The solute carrier 13 (SLC13) family comprises electrogenic sodium ion–coupled anion cotransporters, segregating into sodium ion–sulfate cotransporters (NaSs) and sodium ion–di- and–tricarboxylate cotransporters (NaDCs). NaS1 and NaDC1 regulate sulfate homeostasis and oxidative metabolism, respectively. From an overall view, both the NaDC1 and NaS1 form a homodimer, and each protomer consists of 11 TMDs. The rest TMDs form the core domain that is responsible for substrate recognition and conformational change to complete the transport cycle.

In addition, we elucidated NaDC1’s outward-facing conformation, encompassing apo, citrate-bound, and N-(p-amylcinnamoyl) anthranilic acid (ACA) inhibitor–bound states. NaDC1, a representative member of SLC13 family, mediates both pH-independent, sodium-dependent cotransport of succinate and pH- and sodium-dependent cotransport of citrate within the kidney and small intestine. Citrate molecules are located in the interface of scaffold and core domain. (D) Key residues participating in citrate and sodium binding are from L5, L10, HPin, and HPout of NaDC1. Two bulks of ion densities can be determined in the cryo-EM map, locating in the Na1 and Na2 sites of NaDC1. Na1’s coordination involves the carbonyl oxygen atoms of Ser136 and Ile139, along with the side chain of Asn141 from HPin, and the carbonyl oxygen atoms of Gly239 on L5. Similarly, Na2’s coordination entails the carbonyl oxygen atoms of Thr471 and Thr474, alongside the side chain of Asn476 from HPout, and the carbonyl oxygen atoms of Ala518 on L10. To examine the transport activity, mutations were introduced in NaDC1 by replacing each of these residues with Ala, including the Ser140Ala, Asn141Ala, Thr142Ala, and Asn476Ala. The Tm for WT-NaDC1 is 62.9° ± 0.3°C, while the Tm values are reduced to 57.1° ± 0.7°C for Ser140Ala mutant and 56.4° ± 0.3°C for Thr142Ala, respectively.

>[2x]MADYKDDDDKSGRMATCWQALWAYRSYLIVFFVPILLLPLPILVPSKEAYCAYAIILMALFWCTEALPLAVTALFPLILFPMMGIVDASEVAVEYLKDSNLLFFGGLLVAIAVEHWNLHKRIALRVLLIVGVRPAPLILGFMLVTAFLSMWISNTATSAMMVPIAHAVLDQLHSSQASSNVEEGSNNPTFELQEPSPQKEVTKLDNGQALPVTSASSEGRAHLSQKHLHLTQCMSLCVCYSASIGGIATLTGTAPNLVLQGQINSLFPQNGNVVNFASWFSFAFPTMVILLLLAWLWLQILFLGFNFRKNFGIGEKMQEQQQAAYCVIQTEHRLLGPMTFAEKAISILFVILVLLWFTREPGFFLGWGNLAFPNAKGESMVSDGTVAIFIGIIMFIIPSKFPGLTQDPENPGKLKAPLGLLDWKTVNQKMPWNIVLLLGGGYALAKGSERSGLSEWLGNKLTPLQSVPAPAIAIILSLLVATFTECTSNVATTTIFLPILASMAQAICLHPLYVMLPCTLATSLAFMLPVATPPNAIVFSFGDLKVLDMARAGFLLNIIGVLVIALAINSWGIPLFSLHSFPSWAQSNTTAQCLPSLANTTTPSP> SPPKRLTREAMRNYLKERGDQTVLILHAKVAQKSYGNEKRFFCPPPCVYLMGSGWKKKKEQMERDGCSEQESQPCAFIGIGNSDQEMQQLNLEGKNYCTAKTLYISDSDKRKHFMLSVKMFYGNSDDIGVFLSKRIKVISKPSKKKQSLKNADLCIASGTKVALFNRLRSQTVSTRYLHVEGGNFHASSQQWGAFYIHLLDDDESEGEEFTVRDGYIHYGQTVKLVCSVTGMALPRLIIRKVDKQTALLDADDPVSQLHKCAFYLKDTERMYLCLSQERIIQFQATPCPKEQNKEMINDGASWTIISTDKAEYTFYEGMGPVLAPVTPVPVVESLQLN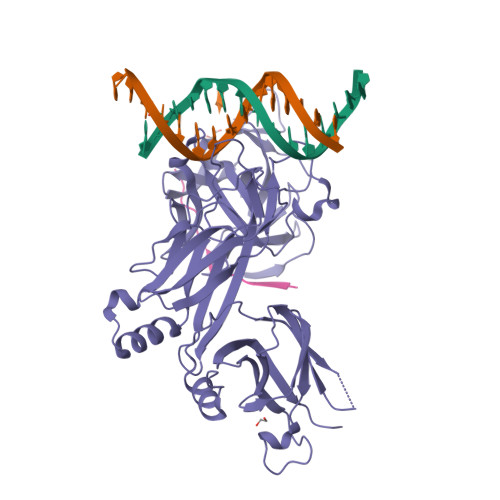GGGDVAMLELTGQNFTPNLRVWFGDVEAETMYRCGESMLCVVPDISAFREGWRWVRQPVQVPVTLVRNDGVIYSTSLTFTYTPEP;> KKATATTTWMVPTA> AGAGQSNDSGIVQQQSNLLRAIEAQQHLLQLTVWGIKQLQTRVLGGGGRWMQWDKEISNYTNTV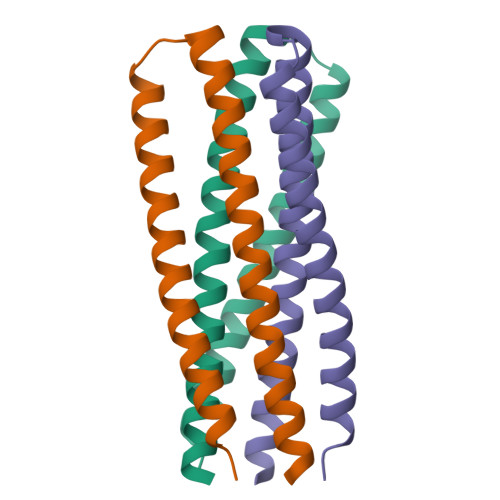YRLLEESQNQQERNEKDLLALA>PVMKTFKEFLLSLDDSVDETEAVKRYNDYKLDFRRQQMQDFFLAHKDEEWFRSKYHPDEVGKRRQEARGALQNRLRVFLSLMETGWFDNLLLDIDKADAIVKMLDAAVIKMEGGTENDLRILEQ[2x];>[2x]GLECKPRPLHKTCSLFMRNIAPNISRAEIISLCKRYPGFMRVALSEPQPERRFFRRGWVTFDRSVNIKEICWNLQNIRLRECELSPGVNRDLTRRVRNINGITQHKQIVRNDIKLAAKLIHTLDDRTQLWASEPGTPPLPTSLPSQNPILKNITDYLIEEVSAEEEELLGSSGGAPPEEPPKEGNPAEINVERDEKLIKVLDKLLLYLRIVHSLDYYNTCEYPNEDEMPNRCGIIHVRGPMPPNRISHGEV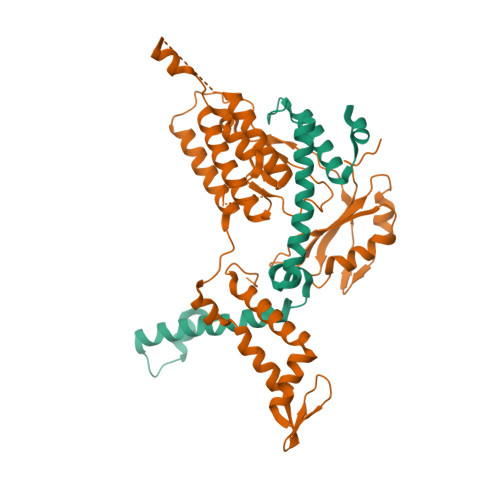LEWQKTFEEKLTPLLSVRESLSEEEAQKMGRKDPEQEVEKFVTSNTQELGKDKWLCPLSGKKFKGPEFVRKHIFNKHAEKIEEVKKEVAFFNNFLTDAKRPALPE>GGGRELSASNSDNVSPVTKSVAFSDRIESSPIYRIPGSSPKPSPSSKPGKSILRNRLPSVRTVSDLSYNKLQYTQHKLHNGNIFTSPYKETRVNPRALEYWVSGEIHGLVDNESVSEFKEIIEGGLGILRQESEDYVARRFEVYATFNNIIPILTTKNVNEVDQKFNILIVNIESIIEICIPHLQIAQDTLLSSSEKKNPFVIRLYVQIVRFFSAIMSNFKIVKWLTKRPDLVNKLKVIYRWTTGALRNENSNKIIITAQVSFLRDEKFGTFFLSNEEIKP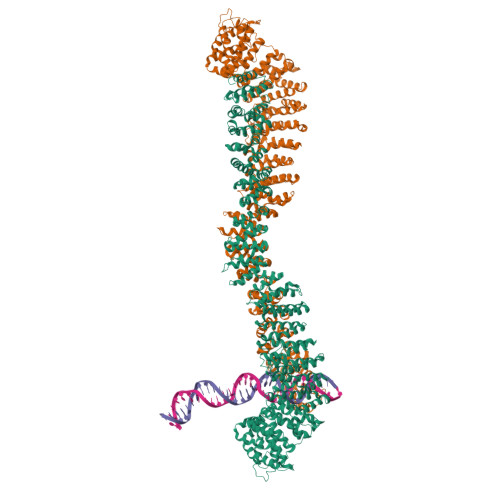IISTFTEIMEINSHNLIYEKLLLIRGFLSKYPKLMIETVTSWLPGEVLPRIIIGDEIYSMKILITSIVVLLELLKKCLDFVDEHERIYQCIMLSPVCETIPEKFLSKLPLNSYDSANLDKVTIGHLLTQQIKNYIVVKNDNKIAMDLWLSMTGLLYDSGKRVYDLTSESNKVWFDLNNLCFINNHPKTRLMSIKVWRIITYCICTKISQKNQEGNKSLLSLLRTPFQMTLPYVNDPSAREGIIYHLLGVVYTAFTSNKNLSTDMFELFWDHLITPIYEDYVFKYDSIHLQNVLFTVLHLLIGGKNADVALERKYKKHIHPMSVIASEGVKLKDISSLPPQIIKREYDKIMKVVFQAVEVAISNVNLAHDLILTSLKHLPEDRKDQTHLESFSSLILKVTQNNKDTPIFRDFFGAVTSSFVYTFLDLFLRKNDSSLVNFNIQISKVGISQGNMTLDLLKDVIRKARNETSEFLIIEKFLELDDKKTEVYAQNWVGSTLLPPNISFREFQSLANIVNKVPNENSIENFLDLCLKLSFPVNLFTLLHVSMWSNNNFIYFIQSYVSKNENKLNVDLITLLKTSLPGNPELFSGLLPFLRRNKFMDILEYCIHSNPNLLNSIPDLNSDLLLKLLPRSRASYFAANIKLFKCSEQLTLVRWLLKGQQLEQLNQNFSEIENVLQNASDSELEKSEIIRELLHLAMANPIEPLFSGLLNFCIKNNMADHLDEFCGNMTSEVLFKISPELLLKLLTYKEKPNGKLLAAVIEKIENGDDDYILELLEKIIIQKEIQILEKLKEPLLVFFLNPVSSNMQKHKKSTNMLRELVLLYLTKPLSRSAAKKFFSMLISILPPNPNYQTIDMVNLLIDLIKSHNRKFKDKRTYNATLKTIGKWIQESGVVHQGDSSKEIEAIPDTKSMYIPCEGSENKLSNLQRKVDSQDIQVPATQGMKE[2x]>[2x]MGHHHHHHSHMGSEIGTGFPFDPHYVEVLGERMHYVDVGPRDGTPVLFLHGNPTSSYLWRNIIPHVAPSHRCIAPDLIGMGKSDKPDLDYFFDDHVRYLDAFIEALGLEEVVLVIHDWGSALGFHWAKRNPERVKGIACMEFIRPIPTWDEWPEFARETFQAFRTADVGRELIIDQNAFIEGALPMGVVRPLTEVEMDHYREPFLKPVDREPLWRLPNELPIAGE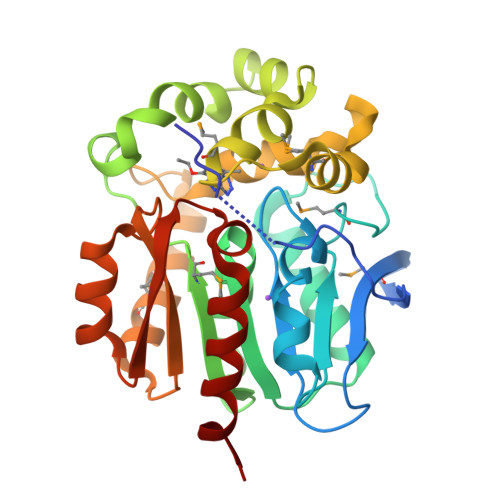PANIVALVEAYMNWLHQSPVPKLLFWGTPGVLIPPAEAARLAESLPNCKTVDIGPGLFLLQEDNPDLIGSEIARWLPGLAG> GMEPEQMLEGQTQVAENPHSEYGLTDNVERIVENEKINAEKSSKQKVDLQSLPTRAYLDQTVVPILLQGL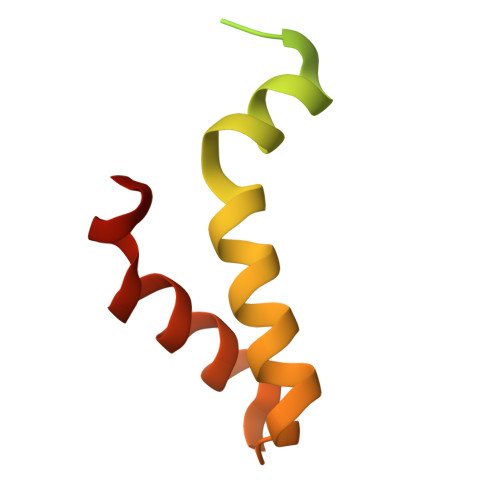AVLAKERPPNPIEFLASYLLKNKAQFEDRN> EDPHLRNRPGKGHNYIDGMTQEDATCKPVTYAGACSSFDVLLEKGKFPLFQSYAHHRTLLEAVHDTIIAKADPPSCDLQSAHGNPCMKEKLVMKTHCPNDYQSAHYLNNDGKMASVKCPPKYELTEDCNFCRQMTGASLKKGSYPLQDLFCQSSEDDGSKLKTKMKGVCEVGVQALKKCDGQLSTAHEVVPFAVFKNSKKVYLDKLDLKTEENLLPDSFVCFEHKGQYKGTMDSGQTKRELKSFDISQCPKIGGHGSKKCTGDAAFCSAYECTAQYANAYCSHANGSGIVQIQVSGVWKKPLCVGYERVVVKRELS

Rift Valley fever virus (RVFV; genus phlebovirus, family Phenuiviridae) is an important example of an enveloped virus that harbours a class II fusion protein. As with other phleboviruses, RVFV displays two glycoproteins on the lipid bilayer envelope of the virion, Gn and Gc, which form higher order pentameric and hexameric ring-shaped assemblies. While the Gc glycoprotein is responsible for membrane fusion, the role of the Gn remains undefined. Virus entry is completed upon Gc-mediated fusion of the viral envelope and host cell membrane, in a pH-dependent mechanism.

We solved the crystal structure of RVFV Gn to 1.6-Å resolution. Although, residues 154–560 were present in the RVFV Gn construct, electron density corresponding to only residues 154–469 was observed, indicating that the remaining 91 C-terminal residues were likely cleaved during crystallogenesis. RVFV Gn adopts a novel fold comprising 15 β-strands, 5 α-helices and 4 310-helices. The protein can be divided into three domains: a predominantly helical N-terminal domain termed ‘domain A’ (residues 154–305), a β-ribbon domain (residues 306–365 and 440–469) and a small globular domain termed ‘B’ (residues 366–439). Superposition analysis revealed a high level of structural similarity between that Gn structure and the one reported in this study (0.4 Å root-mean square deviation between 261 pairs of C-alpha atoms, respectively).>[44x]MSVLTKAIVNADAEARYLSPGELDRIKSFVASGERRLRIAQTLTEARERIVKQAGDQLFQIRPDVVSPGGNAYGEKMTALCLRDLDYYLRLVTYGIVAGDVTPIEEIGIIGVKEMYNSLQTPIPAVAEGVRAMKNVATSLLSGDDAAEAGFYFDYLVGAMQ;>[48x]MQDAITAVINNYDVQGKYLDGAALDKLKAYFTTGAVRVRAAAVISSNATTIIKEAAAKALIYSDLTRPGGNMYTTRRYAACIRDMDYFLRYATYAMLAGDPSILDERVLNGLKETYNSLGVPIAATVGGIQAMKEVVGGLVGPDAAKEASIYFDYLSSGLS;>MSVVLTTIMNADQQLRYPSVGELEQIKNFMEDSALRLKVAKTLSDANDRVVKQASAGLFQRRPDLNNPGGNAYGEKRLGSCIRDL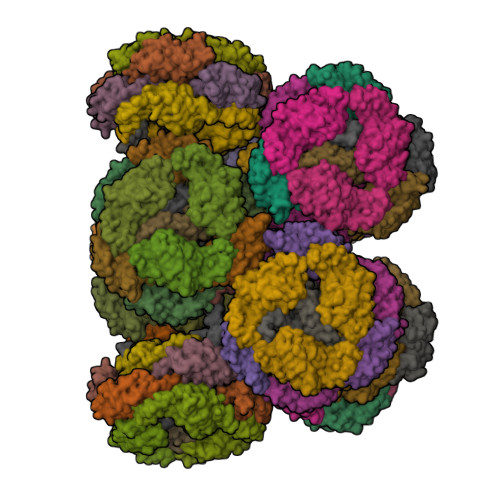GWYYRLITYSIVAGNNEPVERIGLTGIFEMYRVLEVPIPAMIESMRLLKKEALELLSPAEAEIAAPYFDYVIGAMQ[2x];>MSRYFKVTACIPSLKRVRTGRELQNTFFTKLVPYENWFTEQQRIQKAGGKVLSVKLFTGVQGANTGVGA[8x];>MSIRGTSGSTVARPRLFRTVMTETINGINAEDRYPNSGEVSQLDQFFGDGQRRIAIVAKLTENAEMIVSRAANRIFVGGSPMAYSERQKAKAKSPLANDEFGNEPIVEDRGGFLESLKSIFSTRGGGGRASADFAVPPDFEPINIARYGPERMQKSIRDLDWFLRYTTYAILAGDPSILEANCLGLREILEKSCSISATIVALLEMRKNAARLFKDEADSKLVSSYISVVIRALDADRSDAPADIVRPSSEDRPGLTLPYIYKLSADSLTTFKMTAIYGADGRPKVNLSSDEKERVVRAAYRQVFERDLKAYGQSVSEAESKVKNGEISVREFVRRLGKSELYRREFYQPFINSRVLELAFKHFLGRAPESRAEVQKYFSIISSPIVRGQSSMPSGGLYALIDALIDSEEYTSIFGEDTVPYLRNLGVEAQPSWNWGAAYDLYNYAAPRRKVPQFITLFADYTQPLPNQHPYGAGNDPLEIQFGAIFKNSTINPAERAAPIGKDVKRILIRNGSPTSNERGNPTGMSEGATTLGPKIFKLTQNVGFRSKGMVQNAGVVTVEGSVQALITAAYQQIFGRQLYQGQRLKVAEIKLENGETTVKEFVRALGRSEIFRKLYWEPFYVCKAIEYIHRRLLGRPTYDRVENNRYFDIASKKGFYGVVDAMLNSNEYQEVFGEDVLPYERYLTPAGLSLRKGRFGSSDVLTTPGGITPRGDAARMMDKIQELGTPINERSIPEMYVNQGVPALKRQRKVFKQSQATDRESFDALVTAAYVQVFDKDIASYIRSEFSALESRLRNRETSVKEFVRLLGFSALYRKQFHDRYPNTKVVEFAFKHFLGRAVKNQAELIKYHGLLGRKGIKALIGALVDGEEYGRLYGEDTVPSWQFPTLPAANYPNSVELYNRFTRQDDSLVVPSFKPIRSKMDIASMPLVQAALKEQQATKTALDMSRPMFLELGRSFKGADGQSVEVGVGTLRRQLEHIYRIAPDATRSEKDVAINAIYRQVLDVFAGIPPSYLRLSEAESKLKNNEISVREFVRRLGRSENYRKRFFEPYSSPKVVELLTKHFLGRAPISQQEISTYVQILGTKGLAAAVDAIVESPEYLTIFNEDIVPYRRYPTLPAGNYRASVRVNDEELISQSWSSLSPTYTGYQYVTR[2x]>MVMAVNLHKHQKNLVYRLSQQYLAAARDLAADVRSEKQLQQYYTLVRQCVHGLRYVKDGFQLTVEEDIQVTLQLARVLLEETHEVELAEQYLGSLRTRLRTTPLTDARHAVEFQLLYDVPLAKEDRAELRQVVRHTTGLLEELADSDAWAWLFRYCRIIGLEAGGARSNSAVLQEYLKLLQLVSAGPVGLHAFVLCSCVAFILDRVVELDRSLLTQLRALRKAGTAIPLQLQMWSLLLDLLVAIQLDENIMDLLTDFKDFFSTHKDALKDGDDTVVLSIKEGVNVRLFVPLFNYHDCKNILLLFQSVSYLTTCYSKSSNFSTKFLPKVLKTSQELKETLQKRTSLVHVQSIRNIYDKVVDLCRFYQTWESLILSERVEGGIPRLQYSEYNILLEAISSQQAQQADLSHVGRLYSTLTKSKDPELRLIGIAHLYTLIVAELSSCSEGPEGISELTQKTTDAWEQLQHAYLSSSLVQNNVWKCSVAILWAISRFEPFSGHPIHSSSNDQQTLYMQQLNEFFTDNALVGTPEAVPAKDFKLKKSLLLHFLLNYLGGTMLVSDVQKRCDISSSCFQMGKQQYMPGMRYVAGIWHLMNSTVAMKTKEVAITRAKLEGLVDKMLNS[2x];>MSTFPGEDTRIPKRISEALSHQPLNHLVPKRELSRLLSKPVQISVQLESEDAFEEVPEELWQYPHPIDLDPLRLEESQPLRFRRPRGARLDYREDSSEIADLPGMGQLAR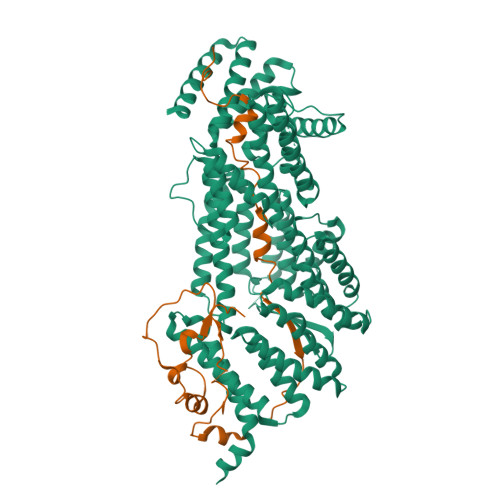ACLSGTQLVDSAAIVESIESNAKKRKQTLAIGDVEMVSPDKKTKVMASVSPVSLNRVALGSQHLKTLERLMQYIGADESSAEFGDFEYWITLEDRATHILSEQCIDKL[2x]>AHAFVSTLTRGDLSSIRWVCSSLRHAQPTCPGAQLCTVYYASLNFRDIMLATGKLSPDAIPGKWTSQDSLLGMEFSGRDASGKRVMGLVPAKGLATSVLLSPDFLWDVPSNWTLEEAASVPVVYSTAYYALVVRGRVRPGETLLIHSGSGGVGQAAIAIALSLGCRVFTTVGSAEKRAYLQARFPQLDSTSFANSRDTSFEQHVLWHTGGKGVDLVLNSLAEEKLQASVRCLATHGRFLEIGKFDLSQNHPLGMAIFLKNVTFHGVLLDAFFNESSADWREVWALVQAGIRDGVVRPLKCTVFHGAQVEDAFRYM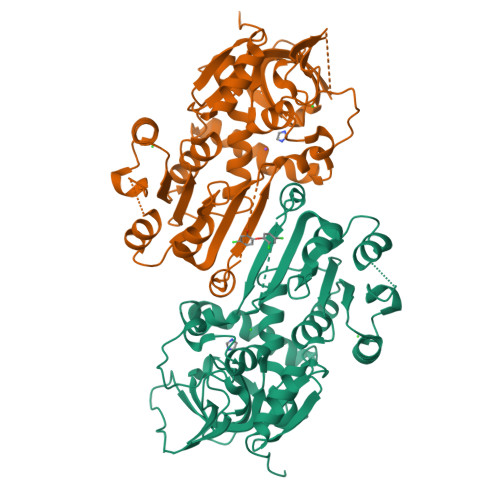AQGKHIGKVVVQVLAEEPEAVLKG[4x]>[2x]GYTLWNDQIVKDEEVKIDKEDRGYQFGDGVYEVVKVYNGEMFTVNEHIDRLYASAEKIRITIPYTKDKFHQLLHELVEKNELNTGHIYFQVTRGTSPRAHQFPENTVKPVIIGYTKENPRPLENLEKGVKATFVEDIRWLRCDIKSLNLLGAVLAKQEAHEKGCYEAILHRNNTVTSGSSSNVFGIKDGILYTHPANNMILKGITRDVVIACANEINMPVKEIPFTTHEALKMDELFVTSTT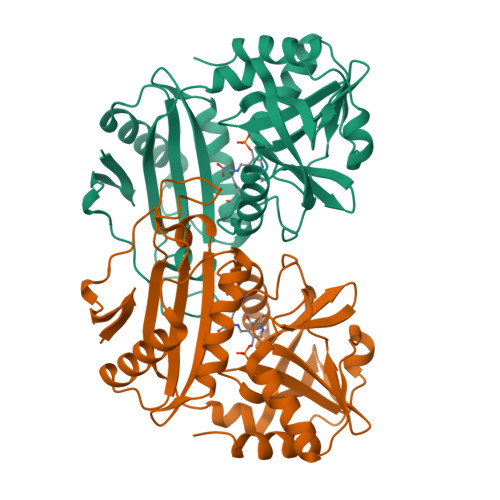SEITPVIEIDGKLIRDGKVGEWTRKLQKQFETKIPKPLHI>MNIPTTTTKGEQAKSQLIAAALAQFGEYGLHATTRDIAALAGQNIAAITYYFGSKEDLYLACAQWIADFLGEKFRPHAEKAERLFSQPAPDRDAIRELILLACKNMIMLLTQEDTVNLSKFISREQLSPTSAYQ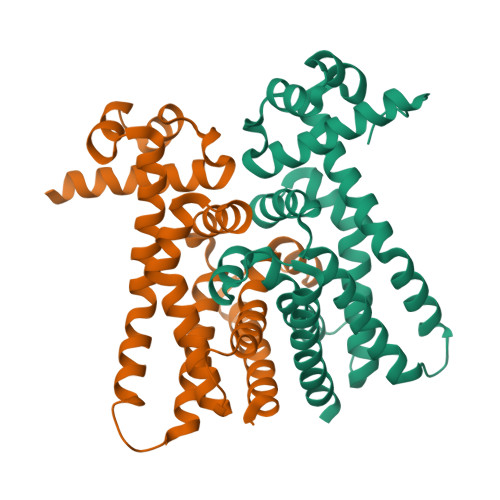LVHEQVIDPLHTHLTRLVAAYTGCDANDTRMILHTHALLGEVLAFRLGKETILLRTGWPQFDEEKAELIYQTVTCHIDLILHGLTQRSLD[2x]> AGLVVNDNDLRNDLAWLSDRGVIHLSLSTWPLSQEEIARALKKAKPSYSSEQVVLARINQRLSALKADFRVTGYTSTDQPGTPQGFGQTQPADNSLGLAFNNSGEWWDVHLQGNVEGGERISNGSRFNANGAYGAVKFWNQWLSFGQVPQWWGPGYEGSLIRGDAMRPMTGFLMQRAEQAAPETWWLRWVGPWQYQISASQMNQYNAVPHAKIIGGRFTFSPIQSLELGASRIMQWGGKGRPESL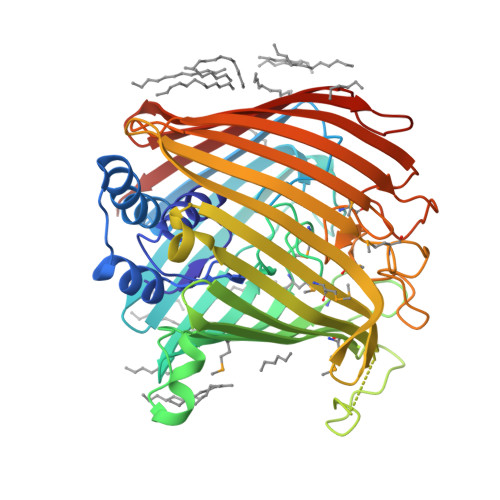SNFWDGLTGKDNTAANDPNEPGNQLAGFDFKFKLEPTLGWPVSFYGQMIGEDESGFLPSANMFLGGIEGHHGWGKDAVNWYLEAHDTRTNMSRTNYSYTHHIYKDGYYQQGYPLGDAMGGDGQLVAGKVELITEDNQRWSTRLVYAKVNPENQSINKAFPHADTLKGIQLGWSGDVYQSVRLNTSLWYTNANNSDSDDVGASAGIEIPFSL> MEQNPQSQLKLLVTRGKEQGYLTYAEVNDHLPEDIVDSDQIEDIIQMINDMGIQVMEEAPDADDLMLAENTADEDAAEAAAQVLSSVESEIGRTTDPVRMYMREMGTVELLTREGEIDIAKRIEDGINQVQCSVAEYPEAITYLLEQYNRVEAEEARLSDLITGFVDPNAEEDLAPTATHVGSELSQEDLDDDEDEDEEDGDDDSADDDNSIDPELAREKFAELRAQYVVTRDTIKAKGRSHATAQEEILKLSEVFKQFRLVPKQFDYVNSMRVMMDRVRTQERLIMKLCVEQCKMPKKNFITLFTGNETSDTWFNAAIAMNKPWSEKLHDVSEEVHRALQKLQQIEEETGLTIEQVKDINRRMSIGEAKARRAKKEMVEANLRLVISIAKKYTNRGLQFLDLI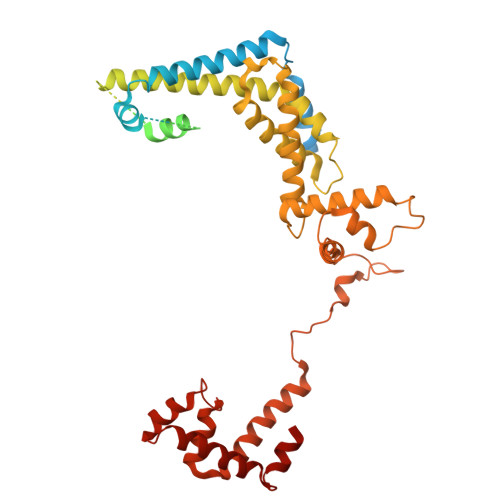QEGNIGLMKAVDKFEYRRGYKFSTYATWWIRQAITRSIADQARTIRIPVHMIETINKLNRISRQMLQEMGREPTPEELAERMLMPEDKIRKVLKIAKEPISMETPIGDDEDSHLGDFIEDTTLELPLDSATTESLRAATHDVLAGLTAREAKVLRMRFGIDMNTDYTLEEVGKQFDVTRERIRQIEAKALRKLRHPSRSEVLRSFLDD NAMPT functions as a homo-dimeric enzyme that catalyzes the rate limiting step in the primary salvage pathway for NAD synthesis, the transfer of a phosphoribosyl residue from 5-phosphoribosyl-1-pyrophosphate (PRPP) to nicotinamide (NAM) to produce nicotinamide mononucleotide (NMN). Crystal structures of NAMPT in numerous ligand-bound forms have been reported. These structures consistently display a NAMPT homo-dimer with two essentially identical active sites at the dimer interface. Typical NAMPT inhibitors were found to occupy the portion of active site responsible for NAM binding and a tunnel-shaped cavity extending from the NAM binding site. Furthermore, we determine the crystal structures of six NAMPT mutants in the apo form and in complex with various inhibitors and present a definitive model to explain the differential effects of the mutations on various structural classes of NAMPT inhibitors.

Unlike the G217A/V mutations, the G217R mutation caused more drastic reduction in the inhibitory potency for all compounds on our test panel. G217R causes His191 side chain to rotate to the same extent as G217V, while introducing additional changes to the structure of the NAMPT inhibitor-binding site. The R217 side chain competes for space with the bound inhibitor (e.g., with the terminal phenyl-trifluoromethyl group of GNE-618) in a similar fashion as H191R. Besides introducing steric clashes, the R217 guanidinium group also creates a basic patch at the surrounding protein surface that favors polar groups over hydrophobic groups. We conclude that these additional structural changes render the G217R mutation more deleterious for NAMPT inhibitor binding across structural classes. In contrast, NCI-H520 cells harboring the G217R mutant are similarly resistant to all 3 NAMPT inhibitors.

>MNPAAEAEFNILLATDSYKVTHYKQYPPNTSKVYSYFECREKKTENSKLRKVKYEETVFYGLQYILNKYLKGKVVTKEKIQEAKDVYKEHFQDDVFNEKGWNYILEKYDGHLPIEIKAVPEGFVIPRGNVLFTVENTDPECYWLTNWIETILVQSWYPITVATNSREQKKILAKYLLETSGNLDGLEYKLHDFGYRGVSSQETAGIGASAHLVNFKRTDTVAGLALIKKYYGTKDPVPGYSVPAAEHSTITAWGKDHEKDAFEHIVTQFSSVPVSVVSDSYDIYNACEKIWGEDLRHLIVSRSTQAPLIIRPDSGNPLDTVLKVLEILGKKFPVTENSKGYKLLPPYLRVIQGDGVDINTLQEIVEGMKQKMWSIENIAFGSGGGLLQKLTRDLLNCSFKCSYVVTNGLGINVFKDPVADPNKRSKKGRLSLHRTPAGNFVTLEEGKGDLEEYGQDLLHTVFKNGKVTKSYSFDEIRKNAQLNIELEAAHHLEHHHHHHHH[2x]> MPLAFCGSENHSAAYRVDQGVLNNGCFVDALNVVPHVFLLFITFPILFIGWGSQSSKVHIHHSTWLHFPGHNLRWILTFMLLFVLVCEIAEGILSDGVTESHHLHLYMPAGMAFMAAVTSVVYYHNIETSNFPKLLIALLVYWTLAFITKTIKFVKFLDHAIGFSQLRFCLTGLLVILYGMLLLVEVNVIRVRRYIFFKTPREVKPPEDLQDLGVRFLQPFVNLLSKGTYWWMNAFIKTAHKKPIDLRAIGKLPIAMRALTNYQRLCEAFDAQVRKDIQGTQGARAIWQALSHAFGRRLVLSSTFRILADLLGFAGPLCIFGIVDHLGKENDVFQPKTQFLGVYFVSSQEFLANAYVLAVLLFLALLLQRTFLQASYYVAIETGINLRGAIQTKIYNKIMHLSTSNLSMGEMTAGQICNLVAIDTNQLMWFFFLCPNLWAMPVQIIVGVILLYYILGVSALIGAAVIILLAPVQYFVATKLSQAQRSTLEYSNERLKQTNEMLRGIKLLKLYAWENIFRTRVETTRRKEMTSLRAFAIYTSISIFMNTAIPIAAVLITFVGHVSFFKEADFSPSVAFASLSLFHILVTPLFLLSSVVRSTVKALVSVQKLSEFLSSAEIREEQCAPHEPTPQGPASKYQAVPLRVVNRKRPAREDCRGLTGPLQSLVPSADGDADNCCVQIMGGYFTWTPDGIPTLSNITIRIPRGQLTMIVGQVGCGKSSLLLAALGEMQKVSGAVFWSSLPDSEIGEDPSPERETATDLDIRKRGPVAYASQKPWLLNATVEENIIFESPFNKQRYKMVIEACSLQPDIDILPHGDQTQIGERGINLSGGQRQRISVARALYQHANVVFLDDPFSALDIHLSDHLMQAGILELLRDDKRTVV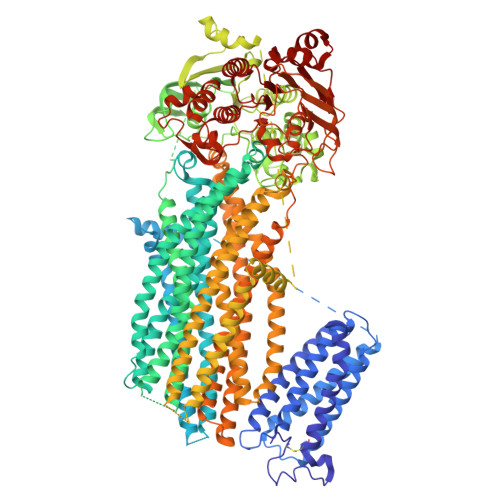LVTHKLQYLPHADWIIAMKDGTIQREGTLKDFQRSECQLFEHWKTLMNRQDQELEKETVTERKATEPPQGLSRAMSSRDGLLQDEEEEEEEAAESEEDDNLSSMLHQRAEIPWRACAKYLSSAGILLLSLLVFSQLLKHMVLVAIDYWLAKWTDSALTLTPAARNCSLSQECTLDQTVYAMVFTVLCSLGIVLCLVTSVTVEWTGLKVAKRLHRSLLNRIILAPMRFFETTPLGSILNRFSSDCNTIDQHIPSTLECLSRSTLLCVSALAVISYVTPVFLVALLPLAIVCYFIQKYFRVASRDLQQLDDTTQLPLLSHFAETVEGLTTIRAFRYEARFQQKLLEYTDSNNIASLFLTAANRWLEVRMEYIGACVVLIAAVTSISNSLHRELSAGLVGLGLTYALMVSNYLNWMVRNLADMELQLGAVKRIHGLLKTEAESYEGLLAPSLIPKNWPDQGKIQIQNLSVRYDSSLKPVLKHVNALIAPGQKIGICGRTGSGKSSFSLAFFRMVDTFEGHIIIDGIDIAKLPLHTLRSRLSIILQDPVLFSGTIRFNLDPERKCSDSTLWEALEIAQLKLVVKALPGGLDAIITEGGENFSQGQRQLFCLARAFVRKTSIFIMDEATASIDMATENILQKVVMTAFADRTVVTIAHRVHTILSADLVIVLKRGAILEFDKPEKLLSRKDSVFASFVRADK> MASHLASIYGTEQDKVNCSFYYKIGACRHGERCSRKHVKPNFSQTILCPNMYKNPIHEPNGKKFTQRELAEQFDAFYEDMFCEFSKYGEVEQLVVCDNVGDHLVGNVYVRFKYEESAQNAIDDLNSRWYSQRPVYAELSPVTDFREACCRQHETSECQRGGLC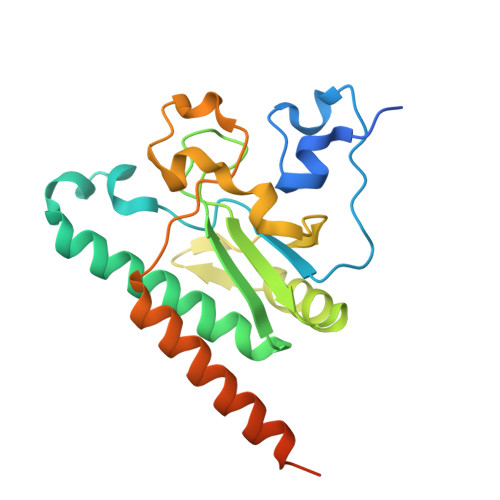NFMHAKKPSPQLLRDLVLAQRKYLALNAAEEMKKEPNSDSTNRWVSVTAERKN> SEVSDTNLYSPFKPRNYQLELALPAMKGKNTIICAPTGCGKTFVSLLICEHHLKKFPQGQKGKVVFFANQIPVYEQNKSVFSKYFERHGYRVTGISGATAENVPVEQIVENNDIIILTPQILVNNLKKGTIPSLSIFTLMIFDECHNTSKQHPYNMIMFNYLDQKLGGSSGPLPQVIGLTASVGVGDAKTTDEALDYICKLCASLDASVIATVKHNLEELEQVVYKPQKFFRKVESRISDKFKYIIAQLMRDTESLAKRICKDLENLSQIQNREFGTQKYEQWIVTVQKACMVFQMPDKDEESRICKALFLYTSHLRKYNDALIISEHARMKDALDYLKDFFSNVRAAGFDEIEQDLTQRFEEKLQELESVSRDPSNENPKLEDLCFILQEEYHLNPETITILFVKTRALVDALKNWIEGNPKLSFLKPGILTGRGKTNQNTGMTLPAQKCILDAFKASGDHNILIATSVADEGIDIAQCNLVILYEYVGNVIKMIQTRGRGRARGSKCFLLTSNAGVIEKEQINMYKEKMMNDSILRLQTWDEAVFREKILHIQTHEKFIRDSQEKPKPVPDKENKKLLCRKCKALACYTADVRVIEDCHYTVLGDAFKECFVSRPHPKPKQFSSFEKRAKIFCARQNCSHDWGIHVKYKTFEIPVIKIESFVVED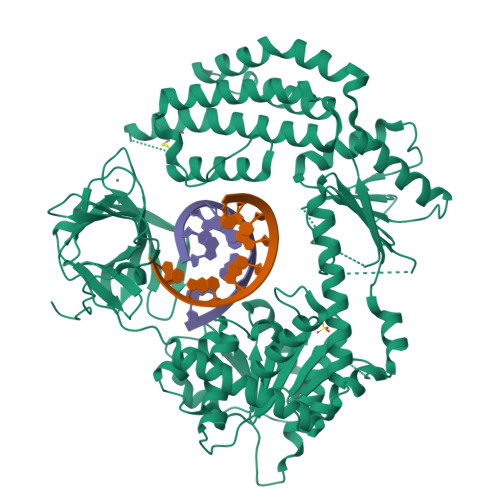IATGVQTLYSKWKDFHFEKIPFDPAEMSK>[2x]MKINDDIKELILEYMSRYFKFENDFYKLPGIKFTDANWQKFKNGGTDIEKMGAARVNAMLDCLFDDFELAMIGKAQTNYYNDNSLKMNMPFYTYYDMFKKQQLLKWLKNNRDDVIGGTGRMYTASGNYIANAYLEVALESSSLGSGSYMLQMRFKDYSKGQEPIPSGRQNRLEWIENNLENIR;> MSDLVLGLDIGIGSVGVGILNKVTGEIIHKNSRIFPAAQAENNLVRRTNRQGRRLTRRKKHRRVRLNRLFEESGLITDFTKISINLNPYQLRVKGLTDELSNEELFIALKNMVKHRGISYLDDASDDGNSSIGDYAQIVKENSKQLETKTPGQIQLERYQTYGQLRGDFTVEKDGKKHRLINVFPTSAYRSEALRILQTQQEFNPQITDEFINRYLEILTGKRKYYHGPGNEKSRTDYGRYRTSGETLDNIFGILIGKCTFYPDEFRAAKASYTAQEFNLLNDLNNLTVPTETKKLSKEQKNQIINYVKNEKAMGPAKLFKYIAKLLSCDVADIKGYRIDKSGKAEIHTFEAYRKMKTLETLDIEQMDRETLDKLAYVLTLNTEREGIQEALEHEFADGSFSQKQVDELVQFRKANSSIFGKGWHNFSVKLMMELIPELYETSEEQMTILTRLGKQKTTSSSNKTKYIDEKLLTEEIYNPVVAKSVRQAIKIVNAAIKEYGDFDNIVIEMARETNEDDEKKAIQKIQKANKDEKDAAMLKAANQYNGKAELPHSVFHGHKQLATKIRLWHQQGERCLYTGKTISIHDLINNSNQFEVDHILPLSITFDDSLANKVLVYATANQEKGQRTPYQALDSMDDAWSFRELKAFVRESKTLSNKK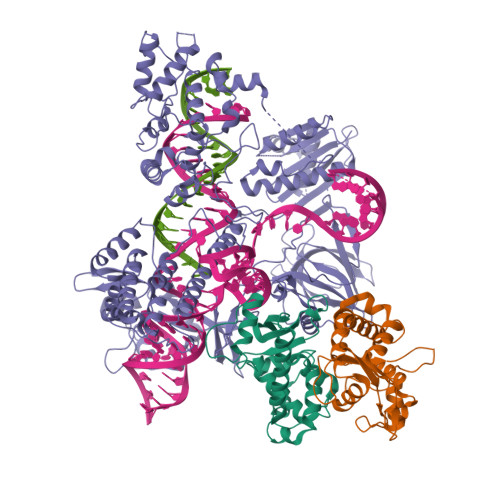KEYLLTEEDISKFDVRKKFIERNLVDTRYASRVVLNALQEHFRAHKIDTKVSVVRGQFTSQLRRHWGIEKTRDTYHHHAVDALIIAASSQLNLWKKQKNTLVSYSEDQLLDIETGELISDDEYKESVFKAPYQHFVDTLKSKEFEDSILFSYQVDSKFNRKISDATIYATRQAKVGKDKADETYVLGKIKDIYTQDGYDAFMKIYKKDKSKFLMYRHDPQTFEKVIEPILENYPNKQINEKGKEVPCNPFLKYKEEHGYIRKYSKKGNGPEIKSLKYYDSKLGNHIDITPKDSNNKVVLQSVSPWRADVYFNKTTGKYEILGLKYADLQFEKGTGTYKISQEKYNDIKKKEGVDSDSEFKFTLYKNDLLLVKDTETKEQQLFRFLSRTMPKQKHYVELKPYDKQKFEGGEALIKVLGNVANSGQCKKGLGKSNISIYKVRTDVLGNQHIIKNEGDKPKLDF> MLRESFAISGDSLISLASTGKRVPIKDLLGEKDFEIWAINEQTMKLESAKVSRVFCTGKKLVYTLKTRLGRTIKATANHRFLTIDGWKRLDELSLKEHIALPRKLESSSLQLAPEIEKLPQSDIYWDPIVSITETGVEEVFDLTVPGLRNFVANDIIVHASIEQDKLGG

Inteins are protein elements that remove themselves from their precursor proteins in an autocatalytic pathway called protein splicing. In the first step of the canonical class 1 inteins, the scissile peptide bond upstream of the intein rearranges in an N–S (or N–O) acyl shift involving the cysteine (or serine) side chain as the first amino acid of the intein (residue 1) and the upstream flanking amino acid of the N-extein (residue (–1)). The M86 mutant of the Ssp DnaB intein (here referred to as WT intein) was selected by sequential directed evolution for its more general activity and is one of the few known intein mutants with improved extein promiscuity.

The importance of steric demand was confirmed by the crystal structure of the M86 precursor intein with the G(–1)F mutation and revealed a constraint imposed around the scissile bond. The sterically demanding Phe side chain in the M86(G(–1)F) mutant is partially squeezed between the His73 imidazole side chain and the N-terminal scissile bond, pushing both moieties slightly apart. The distance between the imidazole ring of the histidine side chain and the amide nitrogen of Ala1 increased from 2.9 Å in the M86 structure (with the π-nitrogen as reference point) to 3.2 or 4.3 Å in the G(–1)F mutant (δ-carbon as reference point), for which two very similar His73 conformers can be observed, indicating increased mobility of this residue. This finding suggests that the polar interaction between the δ-nitrogen of the histidine and the scissile bond amide has been disrupted, at least partially, potentially resulting in a loss of the catalytic contribution of the histidine side chain in case of the M86(G(–1)F) mutant. Consistent with this interpretation is a re-orientation of the His73 imidazole ring, which is flipped in both conformers of the G(–1)F mutant, such that its δ-nitrogen is not facing the amide nitrogen anymore. Instead, the flipped imidazole ring of one of the His73 conformers is stabilized directly by the key Asp136 residue of the block F motif, which also displays a rotated side chain relative to the M86 structure and is within the H-bonding distance of 2.9 Å to the imidazole ring. The flipped orientation of the other His73 conformer in the G(–1)F mutant is assisted by a water molecule (water 145) that is not present in the M86 structure and establishes hydrogen bonds to both the Asp136 side chain and the imidazole moiety. Importantly, the G(–1)F mutation also leads to changes within the backbone geometry around the scissile peptide bond, which expresses itself in changes of the dihedral φ-, ψ- and ω-angles between the (–1) position and Ala1. In the M86(G(–1)F) mutant, the ω-angle (–173°) shows a comparable deviation from the perfect 180° as observed for the WT intein (174°), albeit with an inverted plane.PSTPIP1 is an adaptor protein expressed in most immune cell lineages. It presents two structural domains in its sequence, an N-terminal Fer/CIP4 homology-Bin/Amphiphysin/Rvs (F-BAR) domain and a C-terminal SH3 domain, connected by a linker region. The F-BAR domain of PSTPIP1 binds to the PEST subfamily of protein tyrosine phosphatases (PTPs): PTPN12, also known as PTP-PEST, PTPN18, and the lymphoid phosphatase (LYP), encoded by the gene PTPN22. Positively charged residues on the concave surface of F-BAR domains interact with the polar heads of the phospholipids in the cellular membrane.

To better understand the molecular basis of the physiological function of PSTPIP1 in the immune system, and its role in autoinflammatory diseases, we elucidated the 3D structure of the F-BAR domain (residues 1–289) using X-ray crystallography. Initially, we solved the structure of the G258A mutant, and subsequently that of the wild type protein. The two structures were almost identical. After superimposition, the root mean square deviation (rmsd) between all the equivalent Cα atoms was 0.275 Ǻ, which was similar to the estimated errors of the coordinates of the structures (0.23–0.24 Ǻ). Since the G258A structure was refined to a higher resolution, hereafter, we refer to it. The asymmetric unit of the crystal contains two molecules of PSTPIP1 that form the characteristic elongated crescent-shape of F-BAR dimers. Each protomer consists of five α-helices, with the longer helices, α2, α3, and α4, forming a helical bundle. The dimerization interface is mainly formed by α2, α4, and the shorter helix, α5. Mutations D266N, E277D and D279H, affect acidic residues that are exposed to the solvent on the convex surface but do not make contacts with LYP, and those mutations do not interfere with the interaction. The same is valid for mutations T68M, V122I, G258A and T274M.

>GSHMMPQLQFKDAFWCRDFTAHTGYEVLLQRLLDGRKMCKDMEELLRQRAQAEERYGKELVQIARKAGGQTEINSLRASFDSLKQQMENVGSSHIQLALTLREELRSLEEFRERQKEQRKKYEAVMDRVQKSKLSLYKKAMESKKTYEQKCRDADDAEQAFERISANGHQKQVEKSQNKARQCKDSATEAERVYRQSIAQLEKVRAEWEQEHRTTCEAFQLQEFDRLTILRNALWVHSNQLSMQCVKDDELYEEVRLTLEACSIDADIDSFIQAKSTGTEPPAPVPYQNYYD[2x]>AEPVYPDQLRLFSLGQGVCGDKYRPVNREEAQSVKSNIVGMMGQWQISGLANGWVIMGPGYNGEIKPGTASNTWCYPTNPVTGEIPTLSALDIPDGDEVDVQWRLVHDSANFIKPTSYLAHYLGYAWVGGNHSQYVGEDMDVTRDGDGWVIRGNNDGGCDGYRCGDKTAIKVSNFAYNLDPDSFKHGDVTQSDRQLVKTVVGWAVNDSDTPQSGYDVTLRYDTATNWSKTNTYGLSEKVTTKNKFKWPLVGETELSIEIAANQSWASQNGGSTTTSLSQSVRPTVPARSKIPVKIELYKADISYPYEFKADVSYDLTLSGFLRWGGNAWYTHPDNRPNWNHTFVIGPYKDKAS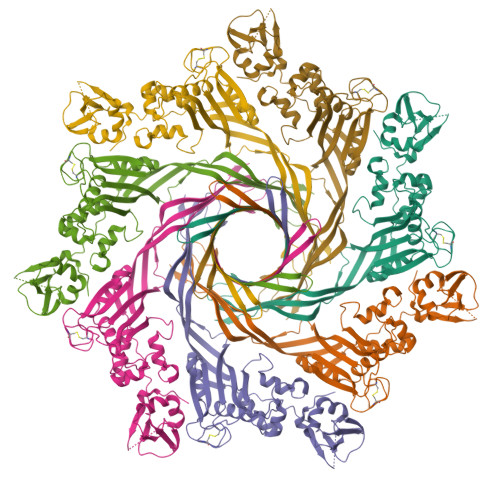SIRYQWDKRYIPGEVKWWDWNWTIQQNGLSTMQNNLARVLRPVRAGITGDFSAESQFAGNIEIGAPVPLAA[7x]(4S)-4-hydroxy-D-proline | C5 H9 N O3 | 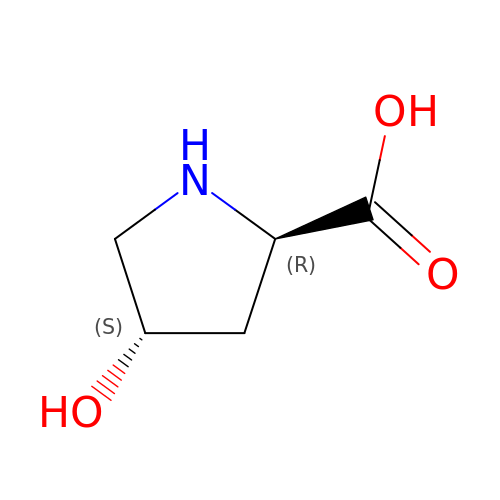PMMYEEVYMWASQN-IUYQGCFVSA-N> MPKLPRGLRFGADNEILNDFQELWFPDLFIESSDTHPWYTLKGRVLNAHLDDRLPNVGGRQVRRTPHRVTVPIASSGLRPVTTVQYDPAALSFLLNARVDWDFGNGDSANLVINDFLFRTFAPKEFDFSNSLVPRYTQAFSAFNAKYGTMIGEGLETIKYLGLLLRRLREGYRAVKRGDLRALRRVIQSYHNGKWKPATAGNLWLEFRYGLMPLFYDIRDVMLDWQNRHDKIQRLLRFSVGHGEDYVVEFDNLYPAVAYFKLKGEITLERRHRHGISYANREGYAVFDNGSLRPVSDWKELATAFINPHEVAWELTPYSFVVDWFLNVGDILAQQGQLYHNIDIVDGFDRRDIRLKSFTIKGERNGRPVNVSASLSAVDLFYSRLHTSNLPFATLDLDTTFSSFKHVLDSIFLLTQRV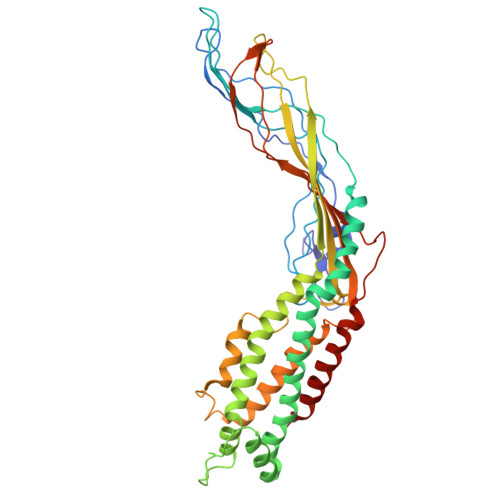KR>[5x]HHHHHHMGKYNLILSEYLSFIYNSQSAVQIPIYYSSNSELENRCIEFHSKCLENSKNGLSLRKLFVEYNDVIENATLLSILSYSYDKYNAVERKLVKYAKGKPLEADLTVNELDYENNKMTSELFPTAEEYTDSLMDPAILTSLSSNLNAVMFWLEKHENDVAEKLKVYKRRLDLFTIVASTINKYGVPRHNAKYRYEYDVMKDKPYYLVTWANSSIEMLMSVFSHDDYLIAKELIVLSYSNRSTLAKLVSSPMSILVALVDINGTFITNEELELEFSNKYVRAIVPDQTFDELNQMLDNMRKAGLVDIPKMIQDWLVDRSIEKFPLMAKIYSWSFHV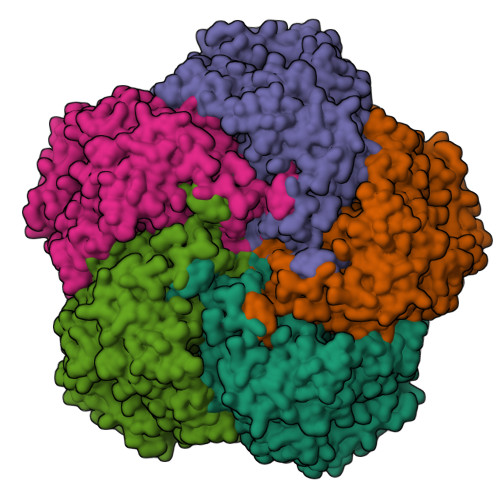GFRKQKMLDAALDQLKTEYTENVDDEMYREYTMLIRDEVVKMLEEPVKHDDHLLRDSELAGLLSMSSASNGESRQLKFGRKTIFSTKKNMHVMDDMANERYTPGIIPPVNVDKPIPLGRRDVPGRRTRIIFILPYEYFIAQHAVVEKMLIYAKHTREYAEFYSQSNQLLSYGDVTRFLSNNTMVLYTDVSQWDSSQHNTQPFRKGIIMGLDILANMTNDAKVLQTLNLYKQTQINLMDSYVQIPDGNVIKKIQYGAVASGEKQTKAANSIANLALIKTVLSRISNKHSFATKIIRVDGDDNYAVLQFNTEVTKQMIQDVSNDVRETYARMNAKVKALVSTVGIEIAKRYIAGGKIFFRAGINLLNNEKRGQSTQWDQAAILYSNYIVNRLRGFETDREFILTKIMQMTSVAITGSLRLFPSERVLTTNSTFKVFDSEDFIIEYGTTVDEVYIQRAFMSLSSQKSGIADEIAASSTFKNYVTRLSEQLLFSKNNIVSRGIALTEKAKLNSYAPISLEKRRAQISALLTMLQKPVTFKSSKITINDILRDIKPFFTVSDAHLPIQYQKFMPTLPDNVQYIIQCIGSRTYQIEDDGSKSAISRLISKYSVYKPSIEELYKVISLHENEIQLYLISLGIPKIDADTYVGSKIYSRDKYRILESYVYNLLSINYGCYQLFDFNSPDLEKLIRIPFKGKIPAVTFILHLYAKLEVINYAIKNGSWISLFCNYPKSEMIKLWKKMWNITSLRSPYTNANFFQEP>[2x]GSAPSVKGVSFDQANNLLIEPARIEEEELTLTILRQTGGLGISIAGGKGSTPYKGDDEGIFISRVSEEGPAARAGVRVGDKLLEVNGVALQGAEHHEAVE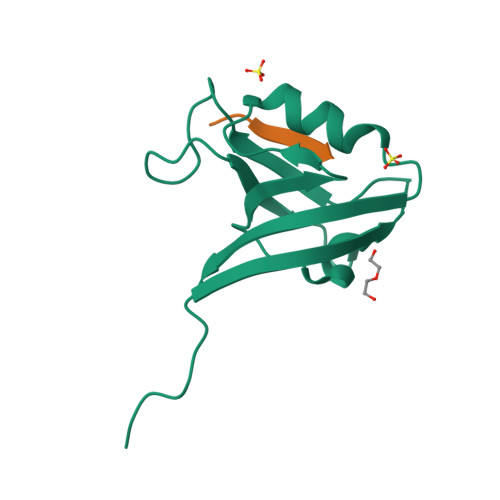ALRGAGTAVQMRVWRERM;>PHTNETSL[2x]6-[(2,5-dimethoxyphenyl)sulfanyl]-3-(1-methyl-1H-pyrazol-4-yl)[1,2,4]triazolo[4,3-b]pyridazine 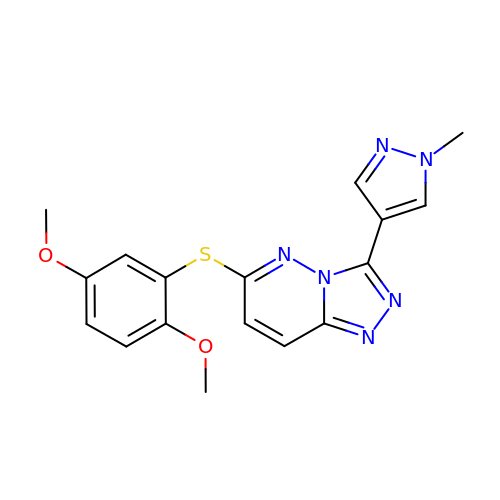| C17 H16 N6 O2 S | RAHGVIZTQAHVRX-UHFFFAOYSA-N6-chloro-4'-[(2-chloro-6-fluorobenzoyl)(methyl)amino]-3'-(2,2,2-trifluoroethoxy)biphenyl-3-carboxamide 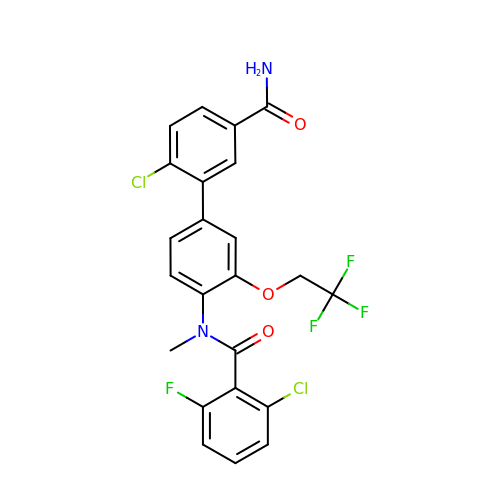| C23 H16 Cl2 F4 N2 O3 | NVMQCZDBIJGVBJ-UHFFFAOYSA-N> IFNGRPAQKGTTPWIAMLSHLNGQPFCGGSLLGSSWIVTAAHCLHQSLDPEDPTLRDSDLLSPSDFKIILGKHWRLRSDENEQHLGVKHTTLHPQYDPNTFENDVALVELLESPVLNAFVMPICLPEGPQQ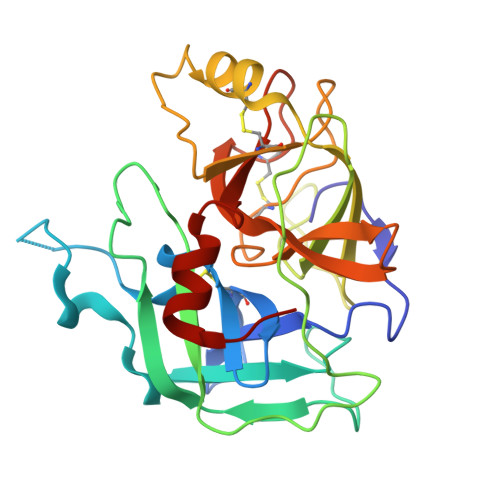EGAMVIVSGWGKQFLQRFPETLMEIEIPIVDHSTCQKAYAPLKKKVTRDMICAGEKEGGKDACAGDSGGPMVTLNRERGQWYLVGTVSWGDDCGKKDRYGVYSYIHHNKDWIQRVTGVRN>MMVLYSGTTCPFSQRCRLVLFEKGMDFEIRDVDLFNKPEDIAVMNPYGQVPILVERDLILYESNIINEYIDERFPHPQLMPADPVQRARARLFLLNFEKELFVHVSTLENEKGKAAEKSHEKARLAIRDRLTQLAPIFLKNKYMLGEEFSMLDVAIAPLLWRLDHYGIELSKNAAPLMKYAERIFSRPAYIEALT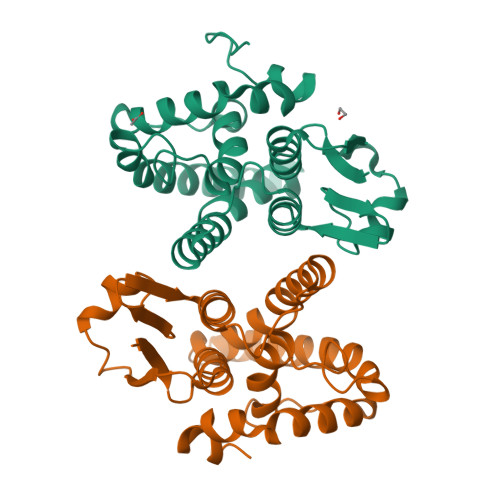PSEKVMRRGHHHHHHH[2x]> GSKDYDELLKYYELHETIGTGGFAKVKLACHILTGEMVAIKIMDKNTLGSDLPRIKTEIEALKNLRHQHICQLYHVLETANKIFMVLEYCPGGELFDYIISQDRLSEEETRVVFRQIVSAVAYVHSQGYAHRDLKPENLLFDEYHKLKLIDFGLCAKPKGNKDYHLQTCCGSLAY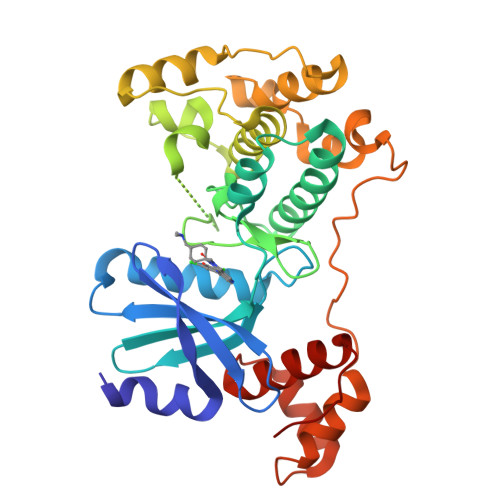AAPELIQGKSYLGSEADVWSMGILLYVLMCGFLPFDDDNVMALYKKIMRGKYDVPKWLSPSSILLLQQMLQVDPKKRISMKNLLNHPWIMQDYNYPVEWQSKNPFIHLDDDCVTELSVHHRNNRQTMEDLISLWQYDHLTATYLLLLAKKARGKPVRLR> GPQSEPELKLESVVIVSRHGVRAPTKATQLMQDVTPDAWPTWPVKLGWLTPRGGELIAYLGHYQRQRLVADGLLAKKGCPQSGQVAIIADVDERTRKTGEAFAAGL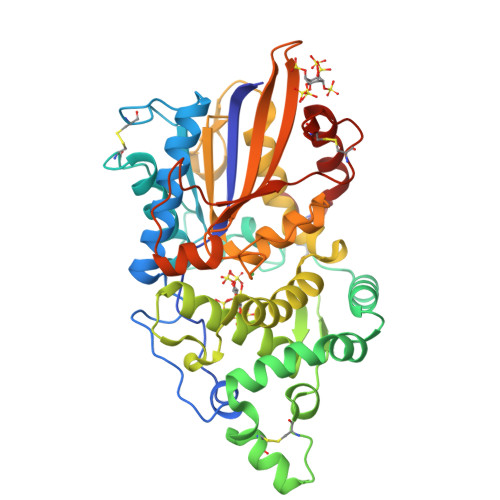APDCAITVHTQADTSSPDPLFNPLKTGVCQLDNANVTDAILSRAGGSIADFTGHRQTAFRELERVLNFPQSNLCLKREKQDESCSLTQALPSELKVSADNVSLTGAVSLASMLTEIFLLQQAQGMPEPGWGRITDSHQWNTLLSLHNAQFYLLQRTPEVARSRATPLLDLIKTALTPHPPQKQAYGVTLPTSVLFIAGHDENLANLGGALELNWTLPGQPDNTPPGGELVFERWRRLSDNSQWIQVSLVFQTLQQMRDKTPLSLNTPPGEVKLTLAGCEERNAQGMCSLAGFTQIVNEARIPACSL>[2x]MAEAGITGTWYNQLGSTFIVTAGADGALT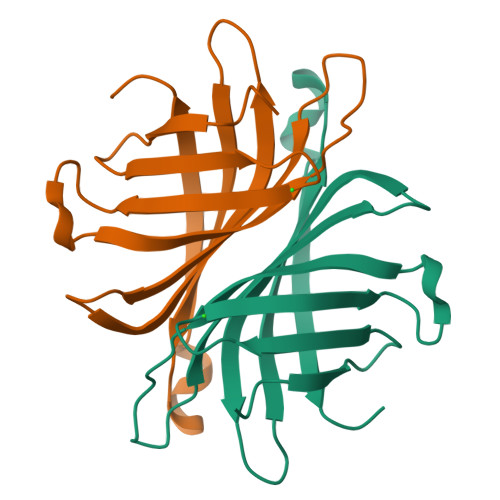GTYESAVGNAESRYVLTGRYDSAPATDGSGTALGWTVAWKNNYRNAHSATTWSGQYVGGAEARINTQWLLTSGTTEANAXKSTLVGHDTFTKVKPSAASLEHHHHHH N-acetyl-L-alpha-aspartyl-L-methionine | C11 H18 N2 O6 S | 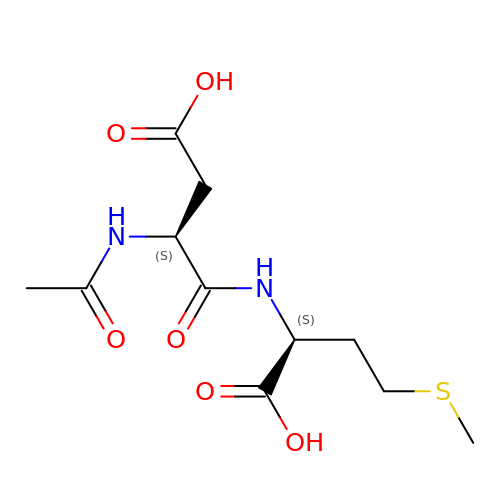FGMUBJQYXOPMHD-YUMQZZPRSA-N> VT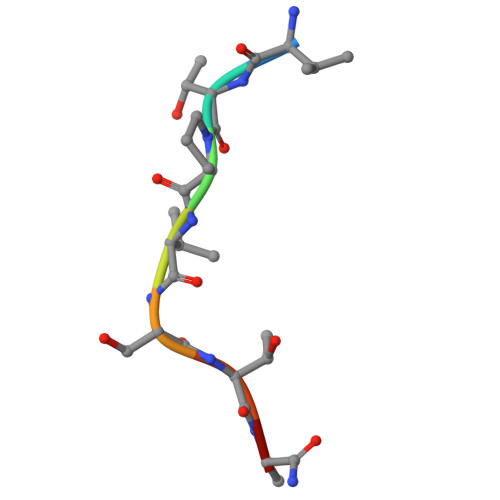PVSTAA>HMASMKKKGSVVIVGRINLSGDTAYAQQTRGEEGCQETSQTGRDKNQVEGEVQIVSTATQTFLATSINGVLWTVYHGAGTRTIASPKGPVTQMYTNVDKDLVGWQAPQGSRSLTPCTCGSSDLYLVTRHADVIPVRRRGDSRGSLLSPRPISYLKGSAGGPLLCPAGHAVGIFRAAVCTRGVAKAVDF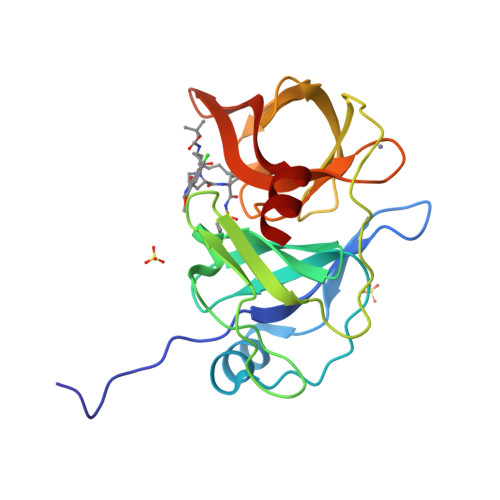IPVESLETTM[2x]> GAMDYSLVKALQTAQQNFVISDPSIPDNPIVYASQGFLTLTGYALSEVLGRNCRFLQGPETDPKAVEKVRKGLERGEDTTVVLLNYRKDGSTFWNQLFIAALRDGEGNVVNYLG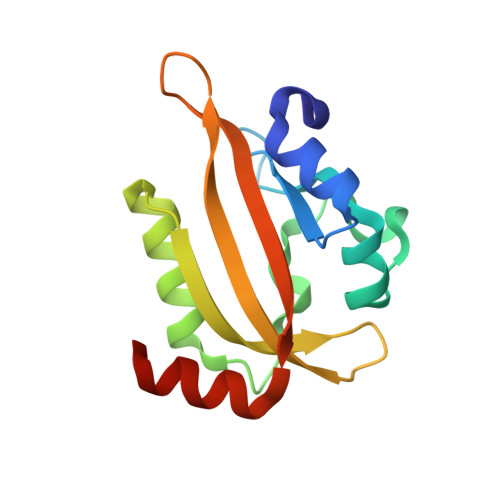VQCKVSEDYAKAFLKNEENE>[12x]MVAPAGEQGRSSTALSDNPFDAKAWRLVDGFDDLTDITYHRHVDDATVRVAFNRPEVRNAFRPHTVDELYRVLDHARMSPDVGVVLLTGNGPSPKDGGWAFCSGGDQRIRGRSGYQYASGDTADTVDVARAGRLHILEVQRLIRFMPKVVICLVNGWAAGGGHSLHVVCDLTLASREYARFKQTDADVGSFDGGYGSAYLARQVGQKFAREIFFLGRTYTAEQMHQMGAVNAVAEHAELET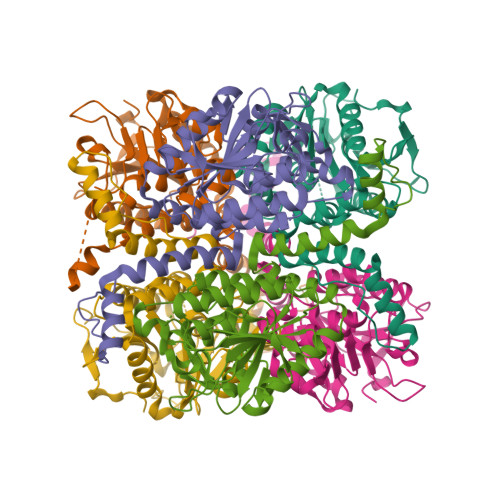VGLQWAAEINAKSPQAQRMLKFAFNLLDDGLVGQQLFAGEATRLAYMTDEAVEGRDAFLQKRPPDWSPFPRYF> MTAQTVTGAVAAAQLGATLPHEHVIFGYPGYAGDVTLGPFDHAAALASCTETARALLARGIQTVVDATPNDCGRNPAFLREVSEA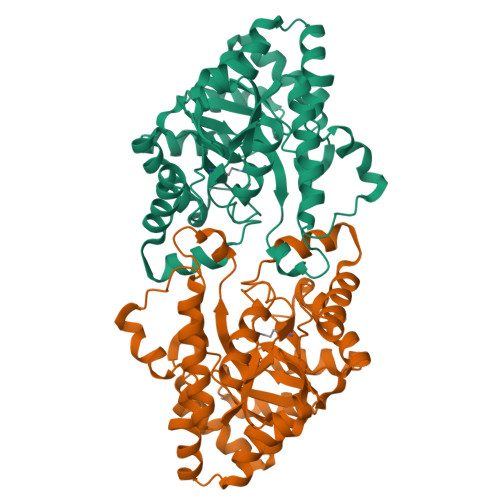TGLQILCATGFYYEGEGATTYFKFRASLGDAESEIYEMMRTEVTEGIAGTGIRAGVIKLASSRDAITPYEQLFFRAAARVQRETGVPIITHTQEGQQGPQQAELLTSLGADPARIMIGHMDGNTDPAYHRETLRHGVSIAFDRIGLQGMVGTPTDAERLSVLTTLLGEGYADRLLLSHDSIWHWLGRPPAIPEAALPAVKDWHPLHISDDILPDLRRRGITEEQVGQMTVGNPARLFG> DKMDYDFKVKLSSERERVEDLFEYEGCKVGRGTYGHVYKAKRKDGKDDKDYALKQIEGTGISMSACREIALLRELKHPNVISLQKVFLSHADRKVWLLFDYAEHDLWHIIKFHRASKANKKPVQLPRGMVKSLLYQILDG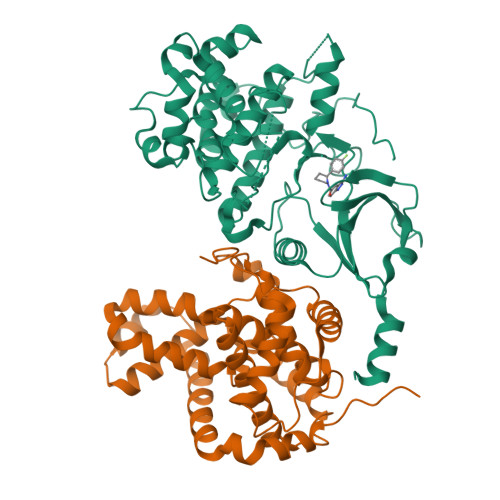IHYLHANWVLHRDLKPANILVMGEGPERGRVKIADMGFARLFNSPLKPLADLDPVVVTFWYRAPELLLGARHYTKAIDIWAIGCIFAELLTSEPIFHCRQEDIKTSNPYHHDQLDRIFNVMGFPADKDWEDIKKMPEHSTLMKDFRRNTYTNCSLIKYMEKHKVKPDSKAFHLLQKLLTMDPIKRITSEQAMQDPYFLEDPLPTSDVFAGCQIPYPKREFLTEEEPPLKK;> DDKAMAGNFWQSSHYLQWILDKQDLLKERQKDLKFLSEEEYWKLQIFFTNVIQALGEHLKLRQQVIATATVYFKRFYARYSLKSIDPVLMAPTCVFLASKVEEFGVVSNTRLIAAATSVLKTRFSYAFPKEFPYRMNHILECEFYLLELMDCCLIVYHPYRPLLQYVQDMGQEDMLLPLAWRIVNDTYRTDLCLLYPPFMIALACLHVACVVQQKDARQWFAELSVDMEKILEIIRVILKLYEQWKNFDERKEMATILSKMPKPKPPP N-(3-{[2-amino-3-(4-phenoxyphenyl)pyridin-4-yl]oxy}phenyl)propanamide 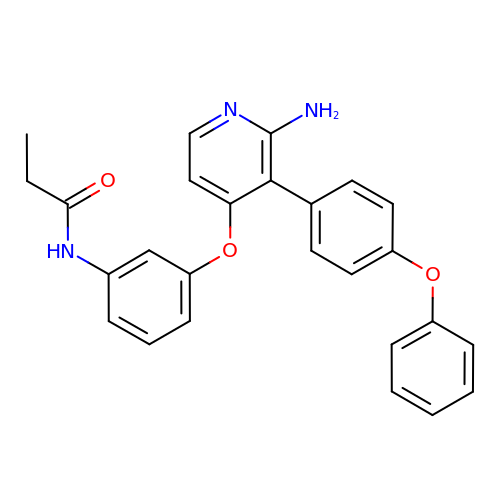| C26 H23 N3 O3 | RTLWGNQEQNXZRG-UHFFFAOYSA-N> 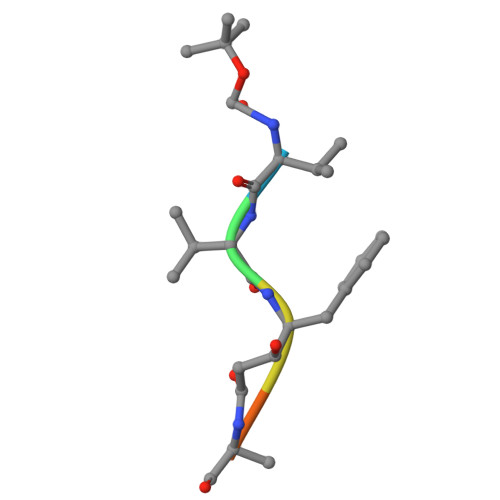VVFAFA N-[(1-methyl-1H-pyrazol-3-yl)methyl]-2-phenylethanamine | C13 H17 N3 | 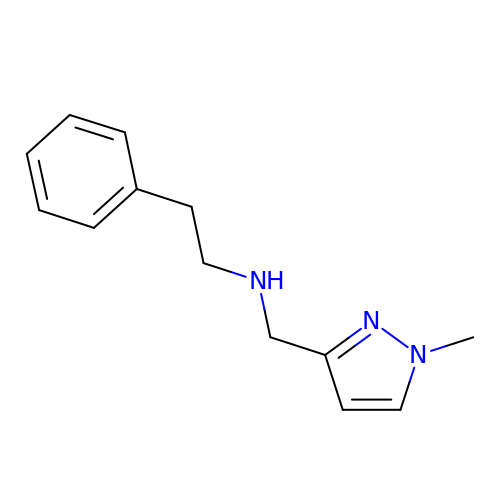KFUQJDBRNAORPV-UHFFFAOYSA-N> PDITHEMGTTSFETTPKKVVALDWVLTETVLSLGIELEGAANISGYQQWVAEPHLNADAIDVGSRREPNLELLSNIKPDVILISKHLAAAYEPLSKIAPVLVYSVYSEDKQPLESAKR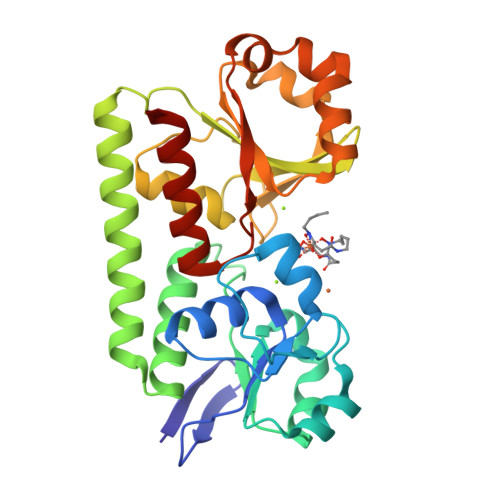ITRSLGKLFDKEQQAEQVIAQTDQRLAANGAKITSAGKAEKPLLFARFINDKTLRIHSEGSLAQDTINAMGLKNDWQEPTNLWGFTTTGTEKLAEHQKANVMIFGPLSQEERQQLTQSPLWQAMEFSRTDSVYELPAIWTFGGLLAAQRLSDHITGRLTQPQ>ADDEDCCSYEDRREIRHIWDDVWSSSFTDRRVAIVRAVFDDLFKHYPTSKALFERVKIDEPESGEFKSHLVRVANGLKLLINLLDDTLVLQSHLGHLADQHIQRKGVTKEYFRGIGEAFARVLPQVLSCFNVDAWNRCFHRLVARIAKDLP[3x];>[3x]KKQCGVLEGLKVKSEWGRAYGSGHDREAFSQAIWRATFAQVPESRSLFKRVHGDDTSHPAFIAHADRVLGGLDIAISTLDQPATLKEELDHLQVQHEGRKIPDNYFDAFKTAILHVVAAQLGRCYDREAWDACIDHIEDGIKGHH;>DEHEHCCSEEDHRIVQKQWDILWRDTESSKIKIGFGRLLLTKLAKDIPEVNDLFKRVDIEHAEGPKFSAHALRILNGLDLAINLLDDPPALDAALDHLAHQHEVREGVQKAHFKKFGEILATGLPQVLDDYDALAWKSCLKGILTKISSRLNA[3x];>[3x]ECLVTESLKVKLQWASAFGHAHERVAFGLELWRDIIDDHPEIKAPFSRVRGDNIYSPEFGAHSQRVLSGLDITISMLDTPDMLAAQLAHLKVQHVERNLKPEFFDIFLKHLLHVLGDRLGTHFDFGAWHDCVDQIIDGIK;> RFQYLVKNQNLHIDYLAKKLHDIEEEYNKLTHDVDKKTIRQLKARISNLEEHHCDEHESECRGDVPECIHDLLFCDGEKDCRDGSDEDPETCSLNITHVGSSYTGLATWTSCEDLNPDHAIVTITAAHRKSFFPNRVWLRATLSYELDEHDHTVSTTQLRGFYNFGKRELLLAPLKGQSEGYGVICDFNLGDDDHADCKIVVPSSLFVCAHFNAQRY;> LDPRLGANAFLIIRLDRIIEKLRTKLDEAEKIDPEHFVSEIDARVEKIEGTHCEKRTFQCGGNEQECISDLLVCDGHKDCHNAHDEDPDVCDTSVVKAGNVFSGTSTWHGCLAREDHVTRITITASKRRKFFTARIWLRALVESELERHGENVTSSFNAKGYYNFASRRLILLPTDDHDDHLAVVCSFNRGDNERAECHRVTEATLHQCADLFVTLEEHD;> QSHDEIIDKIIERTNKITTSISHVESLLDDRLDPKRIRKAGSLRHRVEELEDPSCDEHEHQCGGDDPQCISKLFVCDGHNDCRNGEDEKDCTLPTKAGDKFIGDVCFDHCTKRRPEHMTLAFESSSIAAFFTPIADLHVHIEIESETDEDESEVSMPADGEYSFADHRLTIHPPEEDGLGLVGEFDGYNFDRFVGHIVHELSEEVCAEFIFHRKK

In some invertebrates, including the earthworm L. terrestris, haemoglobins are large extracellular oligomers with D6 point-group symmetry comprised of 144 haem-containing subunits. Giant haemoglobins are arranged as 12 protomers (1/12th units) assembled around a central scaffold of 36 linker chains. Each protomer contains 12 haem groups and possesses a local threefold symmetry axis (which was first revealed by cryo-EM; Schatz et al., 1995) which relates three abcd tetramers to each other. The abcd tetramers themselves have a quasi-C2 symmetry axis, whereby the ad and bc dimers each share a further local dyad axis that is not perpendicular to the quasi-C2 axis of the tetramer.

The structure of the giant haemoglobin from Lumbricus terrestris at a global resolution of ∼3.8 Å is presented as an example of the use of the ABC-4D procedure. We demonstrate our approach using the giant haemoglobin from Lumbricus terrestris as a test sample. This molecule, also known as erythrocruorin, has been a favourite test sample in electron microscopy because of its large size (3.6 MDa) and its ease of specimen preparation. In the present study, the data were acquired in movie mode on a Falcon II camera, resulting in a 3.8 Å resolution map (EMD-3434). Our L. terrestris haemoglobin reconstruction (global FSC resolution of ∼3.8 Å) is comparable in resolution to X-ray crystallography maps. In the best parts of our map the resolution is sufficient to distinguish between large side chains. Some acidic residues have apparently lost side-chain density, which is likely to be a consequence of radiation damage. The most stable part of the map is the linker-chain core of the complex; the haem-containing globins on the outer periphery have a lower resolution owing to flexibility/movement. In our sample many more ‘top views’ than ‘side views’ were present, generating better statistics in the preferred orientation. We conclude that our cryo-EM resolution is in line with the size-related resolutions achieved in X-ray crystallography, and is also primarily limited by the size and flexibilities of the complex. The quasi-atomic environment of a haem group has been elucidated by single-particle cryo-EM for the first time.>MKPQKIVIKLGMPSPKNRTKAMVLAAKVYGVSSVAITGDDKDQLEVVGVDVDTACLVSCLRKKVLRRADIMVVEEAKDK[8x];>GPMQNEYIDAKKHGIDLSRERAPNFVDHPGIPPSDCFWFLYKNYVRQNAGVCQSDWSFDMKIGQYWVTIHTDEGCRLSGIIPAGWLILGMKRPGF[8x]

Here, we unravelled the biochemical and structural basis of adaptive evolution of APikL2, an exceptionally conserved paralog of the well-studied rice-lineage specific effector AVR-Pik. Whereas AVR-Pik and other members of the six-gene AVR-Pik family show specific patterns of presence/absence polymorphisms between grass-specific lineages of M. oryzae, APikL2 stands out by being ubiquitously present in all blast fungus lineages from 13 different host species. Using biochemical, biophysical and structural biology methods, we show that a single aspartate to asparagine polymorphism expands the binding spectrum of APikL2 to host proteins of the heavy-metal associated (HMA) domain family. The structures were solved and refined as described in the Materials and Methods. In each case, the APikL2 variants and HMAs form 1:1 complexes, with both displaying the same global fold and interaction interfaces as previously described for the interaction of AVR-Pik with the Pik-1 integrated HMA domains.

We crystallized complexes of APikL2F with sHMA94 and APikL2A with sHMA25 following co-expression in E. coli for comparative structural analysis. X-ray diffraction data were collected at the Diamond Light Source (Oxford, UK) to 2.3 Å and 1.8 Å resolution, for APikL2F/sHMA94 and APikL2A/sHMA25, respectively. The APikL2F/sHMA94 and APikL2A/sHMA25 complexes display the three binding interfaces previously reported for AVR-Pik/HMA complexes. Consequently, we could only measure binding affinity of APikL2F to sHMA94 with a calculated Kd of 145.8 nM. However, we observed that the presence of Asn-66 in APikL2F results in an altered local hydrogen bonding network around Gln-44 in sHMA94, when compared to Asp-66 in the APikL2A/sHMA25 complex. As a result, the side chain of Gln-44 of sHMA94 is rotated relative to Gln-43 of sHMA25, allowing Gln-44 to form additional intramolecular hydrogen bonds with Thr-38 in sHMA94. In this orientation, the NE2 atom of Gln-44 interacts with the OG1 atom and backbone carbonyl of Thr-38. The altered hydrogen bonding network around Gln-44 in the APikL2F/sHMA94 complex, compared to APikL2A/sHMA25, appears to firmly lock Gln-44 in place compared to Gln-43 of sHMA25. This suggests that the interaction with Asn-66 of APikL2F results in reduced flexibility of the sHMA94 loop in interface 2. Our data indicates that this hydrogen bonding network stabilizes the interaction between APikL2F and sHMA94, providing an explanation for the binding specificity observed in the yeast two-hybrid and in vitro binding affinity assays.> MTSTTPSHPRVRFAPSPTGYLHVGGARTALFNWLYARHTNGTFILRIEDTDASRNTPQALSVIFENLRWLGLDWDEGPLPDGRTIGPFGPYFQSQRNDIYEAYCKKLIDKDMAYIKEGAVLFRMPRKRIIVPDIICGDIYFDCTLEKDFVIRRKDGSFVFHLVNVVDDCEMKISHVIRGEDHLSNTP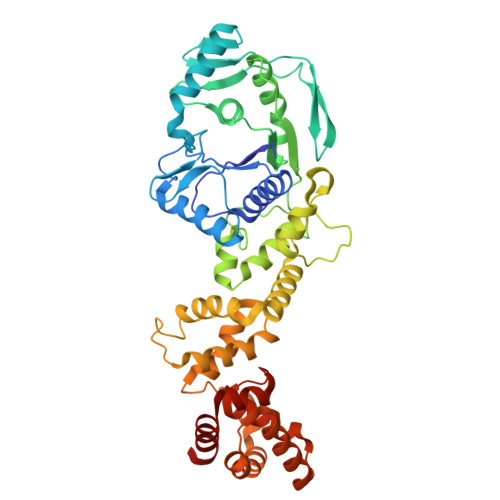KHIAIFESLGIKPPLYAHIPLILNPEGSKMSKRDKGSSVQEYIDEGYLPKAFRNYLCLLGWSIKENREIFDIEEAIAKFDLTQIHRSNARFNRQKLLWLNGEYMRTMPLDELFPHALSWLKKAGLIDDHYDNIPFLKGAVAIVREKVKTGKELIDWIKPLLSNQIEYNDAVLQQYLDNEGKNILKEAFPYLEKVSPFHSKELEETIKSLAMKHGRKTADYIHRLRVALTGRTVGPSLYPMLEVLGKEKVLNRLHKVLFEHE> GAGS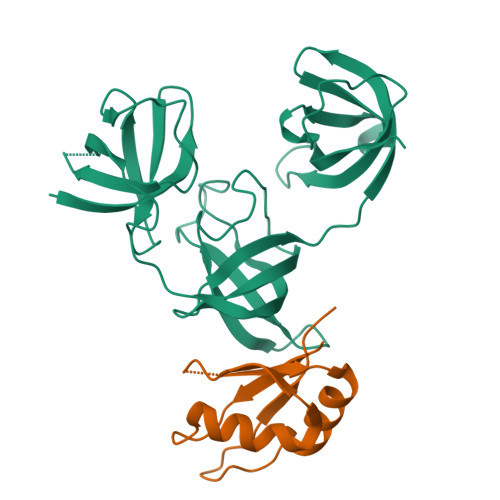DAGQVYRGFIAVMKENFGFIETLSHDEEVFFHFSNYMGNPNWLELGQEVEYTLARNGNTSVSGNCLPAENVRMLPKNSIPQPAVLETTHNGVVARPLRCINPDQQEYAGLIEILDELRTTVISQHEFGITSLVNKRDLLQKGDLVSFRIDESGRAACVNAVRQKKRATVDSIKGQFGFLNFEVEDGKKLFFHMSEVQGNTVALHPGDTVEFSVVTNQRNGKSSACNVLKIND;> GAGEKAKLFTNVYVKNFTEDFDDEKLKEFFEPYGKITSYKVMSKEDGKSKGFGFVAFETTEAAEAAVQALNGKDMGEGKSLYVARAQKKA(2S,6S)-2-amino-6-{[(1E)-{3-hydroxy-2-methyl-5-[(phosphonooxy)methyl]pyridin-4-yl}methylidene]amino}heptanedioic acid | C15 H22 N3 O9 P | 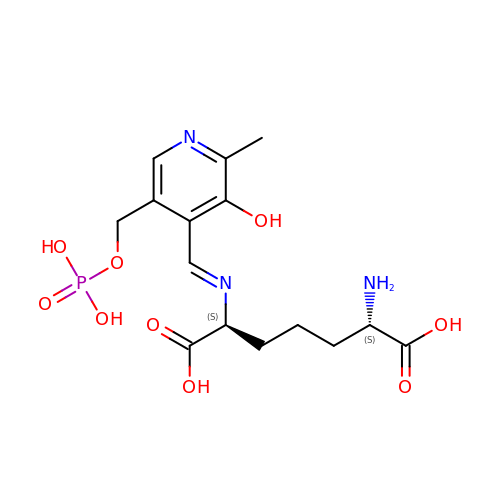VHNMKXLQZMEZSG-NTQSYZAISA-N> GSGGRATMVKLLPAQEAAKIYHTNYVRNSRAVGVMWGTLTICFSVLVMALFIQPYWIGDSVSTPQAGYFGLFSYCVGNVLSSELICKGGP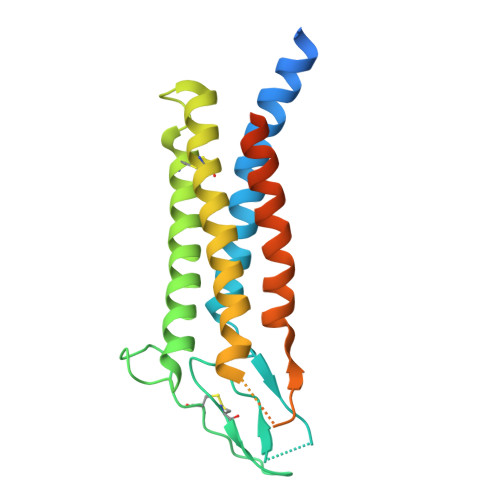LDFSSIPSRAFKTAMFFVALAMFLIIGSIICFSLFFVCNTATVYKICAWMQLAAATGLMIGCLVYPDGWDSSEVRRMCGEQTGKYTLGHCTIRWAFMLAILSIGDALILSFLAFVLGYRQDKLLPDDYKADGNEEVFE2-benzyl-1-phenyl-3-(piperazin-1-ylcarbonyl)-1H-indole 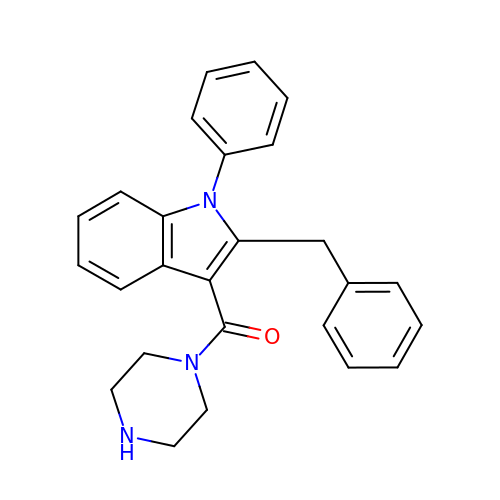| C26 H25 N3 O | FYDPGAJRQXSCCK-UHFFFAOYSA-N> MKVEEILEKALELVIPDEEEVRKGREAEEELRRRLDELGVEYVFVGSYARNTWLKGSLEIDVFLLFPEEFSKEELRERGLEIGKAVLDSYEIRYAEHPYVHGVVKGVEVDVVPCYKLKEPKNIKSAVDRTPFHHKWLEGRIKGKENEVRLLKGFLKANGIYGAEYKVRGFSGYLCELLIVFYGSFLETVKNARRWTRRTVIDVAKGEVRKGEEFFVVDPVDEKRNVAANLSLDNLARFVHLCREFMEAPSLGFFKPKHPLEIEPERLRKIVEERGTAVFAVKFRKPDIVDDNLYPQLERASRKIFEFLERENFMPLRSAFKASEEFCYLLFECQIKEISRVFRRMGPQFEDERNVKKFLSRNRAFRPFIENGRWWAFEMRKFTTPEEGVRSYA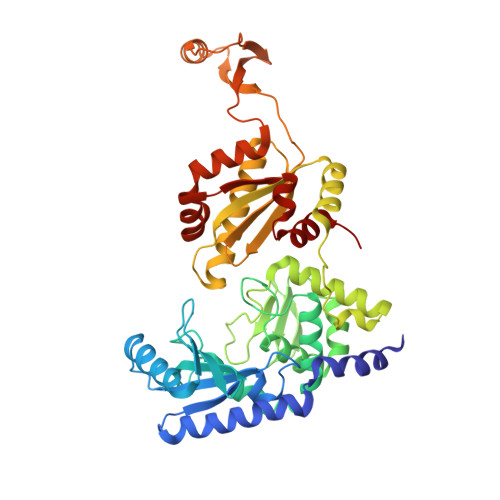STHWHTLGKNVGESIREYFEIISGEKLFKEPVTAELCEMMGVKD>MAKEPVRVLVTGAAGQIGYALVPMIARGIMLGADQPVILHMLDIPPAAEALNGVKMELIDAAFPLLKGVVATT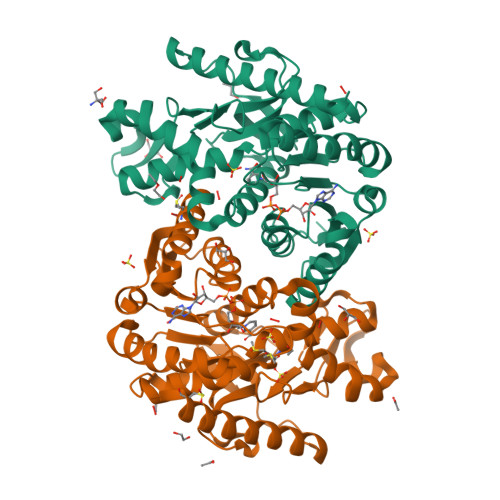DAVEGCTGVNVAVMVGGFPRKEGMERKDVMSKNVSIYKSQAAALEKHAAPNCKVLVVANPANTNALILKEFAPSIPEKNISCLTRLDHNRALGQISERLSVPVSDVKNVIIWGNHSSSQYPDVNHAKVQTSSGEKPVRELVKDDAWLDGEFISTVQQRGAAIIKARKLSSALSAASSACDHIRDWVLGTPEGTFVSMGVYSDGSYSVPSGLIYSFPVTCRNGDWSIVQGLPIDEVSRKKMDLTAEELKEEKDLAYSCLS[3x]> MENTENSVDSKSIKNLEPKIIHGSESMDSGISLDNSYKMDYPEMGLCIIINNKNFHKSTGMTSRSGTDVDAANLRETFRNLKYEVRNKNDLTREEIVELMRDVSKEDHSKRSSFVCVLLSHGEEGIIFGTNGPVDLKKIGNFFRGDRCRSLTGKPKL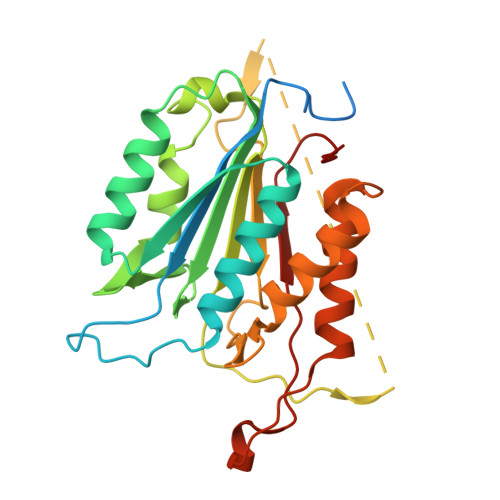FIIQACRGTELDCGIETDSGVDDDMACHKIPVEADFLYAYSTAPGYYSWRNSKDGSWFIQSLCAMLKQYADKLEFMHILTRVNRKVATEFESFSFDATFHAKKQIPCIVSMLTKELYFYH>[2x]ADESVVEPKTGFSFPASIGDSRRLLGVGLRKKSLLGLKNIDVYAFGVYADCDDVKKLVGDKYANLPASEIRGNKSFMDDLMEADIKMTIRLQIVYGKLNIRSVRNAFQESVGN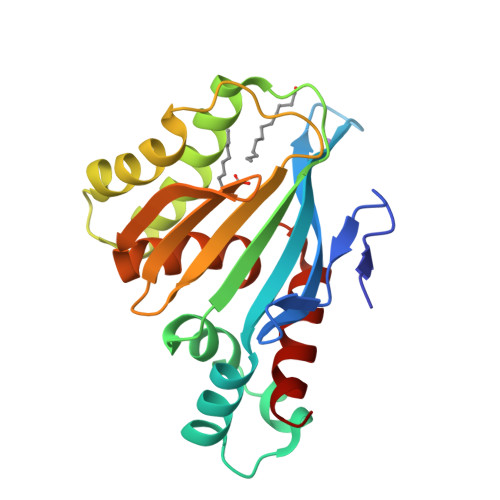RLKKFGGSDNDELLQSFTSLFKDEYKIPRNSTIDLTKDPGHVLSVAIEGNHVGSVKSHLLCRSILDLYIGEEPFDKNAREDFLDNAASLAFD> DTN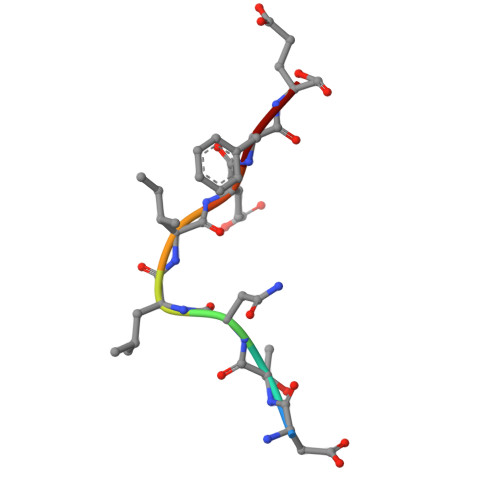LIEFE> NQSVVVDFLLPTGVYLNFPVSRNANLSTIKQLLWHRAQYEPLFHMLSGPEAYVFTCINQTAEQQELEDEQRRLCDVQPFLPVLRLVAREGDRVKKLINSQISLLIGKGLHEFDSLCDPEVNDFRAKMCQFCEEAAARRQQLGWEAWLQYSFPLQLEPSAQTWGPGTLRLPNRALLVNVKFEGSEESFTFQVSTKDVPLALMACALRKKATVFRQPLVEQPEDYTLQVNGRHEYLYGSYPLCQFQYICSCLHSGLTPHLTMVHSSSILAMRDEQSNPAPQVQKPRAKPPPIPAKKPSSVSLWSLEQPFRIELIQGSKVNADERMKLVVQAGLFHGNEMLCKTVSSSEVSVCSEPVWKQRLEFDINICDLPRMARLCFALYAVIEKAKKARSTKKKSKKADCPIAWANLMLFDYKDQLKTGERCLYMWPSVPDEKGELLNPTGTVRSNPNTDSAAALLICLPEVAPHPVYYPALEKILELGRHSECVHVTEEEQLQLREILERRGSGELYEHEKDLVWKLRHEVQEHFPEALARLLLVTKWNKHEDVAQ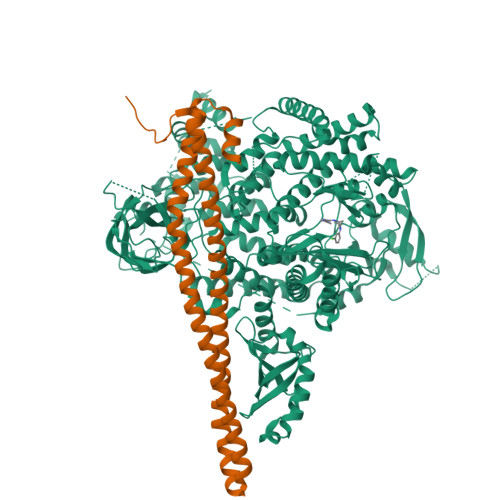MLYLLCSWPELPVLSALELLDFSFPDCHVGSFAIKSLRKLTDDELFQYLLQLVQVLKYESYLDCELTKFLLDRALANRKIGHFLFWHLRSEMHVPSVALRFGLILEAYCRGSTHHMKVLMKQGEALSKLKALNDFVKLSSQKTPKPQTKELMHLCMRQEAYLEALSHLQSPLDPSTLLAEVCVEQCTFMDSKMKPLWIMYSNEEAGSGGSVGIIFKNGDDLRQDMLTLQMIQLMDVLWKQEGLDLRMTPYGCLPTGDRTGLIEVVLRSDTIANIQLNKSNMAATAAFNKDALLNWLKSKNPGEALDRAIEEFTLSCAGYCVATYVLGIGDRHSDNIMIRESGQLFHIDFGHFLGNFKTKFGINRERVPFILTYDFVHVIQQGKTNNSEKFERFRGYCERAYTILRRHGLLFLHLFALMRAAGLPELSCSKDIQYLKDSLALGKTEEEALKHFRVKFNEALRESWKTKV;> YQQDQVVKEDNIEAVGKKLHEYNTQFQEKSREYDRLYEDYTRTSQEIQMKRTAIEAFNETIKIFEEQCQTQERYSKEYIEKFKREGNETEIQRIMHNYEKLKSRISEIVDSRRRLEEDLKKQAAEYREIDKRMNSIKPDLIQLRKTRDQYLMWLTQKGVRQKKLNEWLGN>[4x]HHHHHHEPRPNEECLQILGNAEKGAKFLSDAEIIQLVNAKHIPAYKLETLIETHERGVSIRRQLLSKKLSEPSSLQYLPYRDYNYSLVMGACCENVIGYMPIPVGVAGPLCLDEKEFQVPMATTEGCLVASTNRG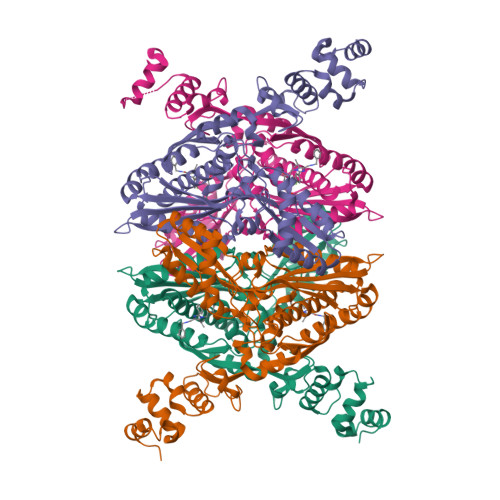CRAIGLGGGASSRVLADGMTRGPVVRLPRACDSAEVKAWLETSEGFAVIKEAFDSTSRFARLQKLHTSIAGRNLYIRFQSRSGDAMGMNMISKGTEKALSKLHEYFPEMQILAVSGNYCTDKKPAAINWIEGRGKSVVCEAVIPAKVVREVLKTTTEAMIEVNINKNLVGSAMAGSIGGYNAHAANIVTAIYIACGQDAAQNVGSSNCITLMEASGPTNEDLYISCTMPSIEIGTVGGGTNLLPQQACLQMLGVQGACKDNPGENARQLARIVCGTVMAGELSLMAALAAGHLVKSHMIHNRSKIN> T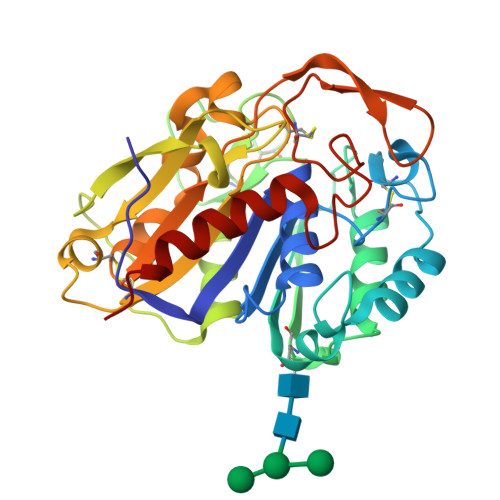ALPAFNVNPNSVSVSGLSSGGYMAAQLGVAYSDVFNVGFGVFAGGPYDCARNQYYTSCMYNGYPSITTPTANMKSWSGNQIASVANLGQRKIYMWTGSSDTTVGPNVMNQLKAQLGNFDNSANVSYVTTTGAVHTFPTDFNGAGDNSCSLSTSPYISNCNYDGAGAALKWIYGSLNARNTGTLSGSVLSFAQSGSYGANGMDTTGYLYVPQSCASGATVCSLHVALHGCLQSYSSIGSRFIQNTGYNKWADTNNMIILYPQAIPDYTIHAIWNGGVLSNPNGCWDWVGWYGSNADQIGGVQMAAIVGQVKQIVSGFQ> GGCAAGGUACGGCG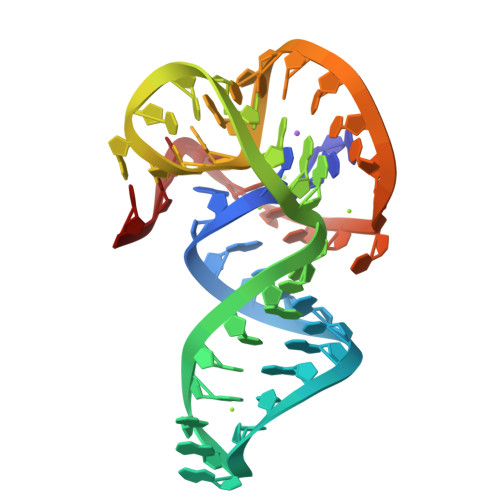AAAGCCGUAGGGGCUUGAGAACCCCCCCUCCCCACUC>MRVGIPTETKNNEFRVAITPAGVAELTRRGHEVLIQAGAGEGSAITDADFKAAGAQLVGTADQVWADADLLLKVKEPIAAEYGRLRHGQILFTFLHLAASRACTDALLDSGTTSIAYETVQTADGALPLLAPMSEVAGRLAAQVGAYHLMRTQGGRGVLMGGVPGVEPADVVVIGAGTAGYNAARIANGMGATVTVLDINIDKLRQLDAEFCGRIHTRYSSAYELEGAVKRADLVIGAVLVPGAKAPKLVSNSLVAHMKPGAVLVDIAIDQGGCFE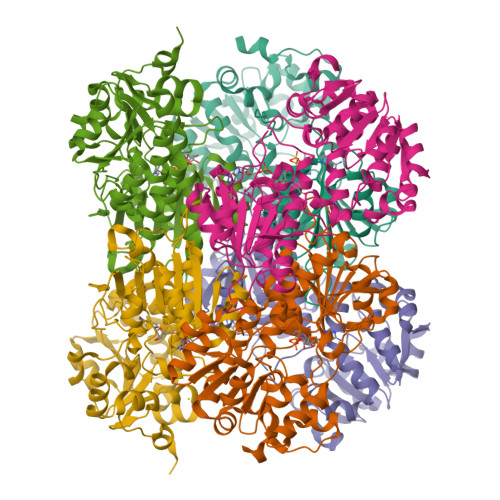GSRPTTYDHPTFAVHDTLFYCVANMPASVPKTSTYALTNATMPYVLELADHGWRAACRSNPALAKGLSTHEGALLSERVATDLGVPFTEPASVLAHHHHHH[6x]>GHHHHHHVGPGSDEVDAPEPPSADYASLVDVFVGTEGDFGNDMPAAQAPNGLAKVNPRTTPGRNNTGYDYAQSKISGFTHTNLDGVGGSGGGGDLLVVPTSGSYTARPGTGTYAHPFSHDDEDAGPGFYSVGLGNVAGTDGAITGAPGTIEAEVAAATRSGVHRYAFPAGSTPSLVVDLETNNTSRRSSSVQVETRADGTVELSGQVTGYFYNAAYTLYYTARTLQPATVQTWGDDDRLVDATAQDGVDTGAILTFDPADAGEIGLQVTLSPVSVEQARIDQQVELGDLSFDAIRDRTRAEWNATLGRVAIDASTATDPTGELQRLFYTHLYRMFAMPMNATSTSGTYRGVDGAVHAAQGFTYYDSWATWDDFRKFSVIAYIDPALYRDMVQSLVYLFADAEATGTGGGLGGFVHSVPTVRWERSSVVVADAIAKGFDGFDRLDEAYPALQRLVGQYSADELRRGYVAGNPGASVQRGYDQYGLSVIADELGLTEEAETLREQASWPIEKLTKPGAWTAADGTQVGLLTPRAADGSWQSADHAKFEAAGLYQGTLWQYHWYDAYDMDALVEAMGGHEAARLGMRHMFGEHAPDDGKAMLHSNANEIDLQAPYLFNYTGEPSLTQKWARAIYTKETWNRYIATGSSSAVPSGGGEFTPPLKTKVYRLDPRGMLPTMDNDAGTMSTMFVAAAVGLFPVTAGSSQFQVGSPFFDSTTITYDDGSAFTVTADGVSEDAFYVQ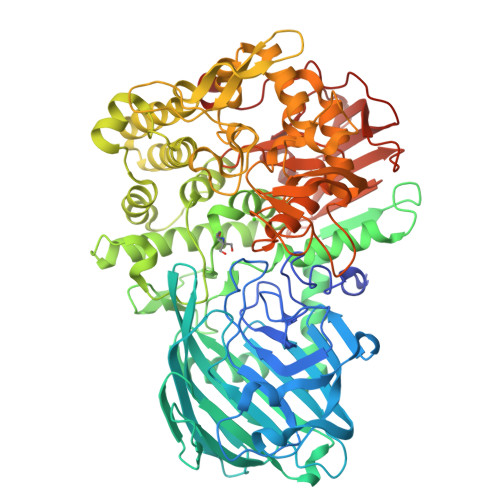SATLDGATFGNTWVDYATVVGGADLAFRMGEQPSDWGTDTAPAFSMSTATDE[2x]2-(4-METHYL-THIAZOL-5-YL)-ETHANOL | C6 H9 N O S | 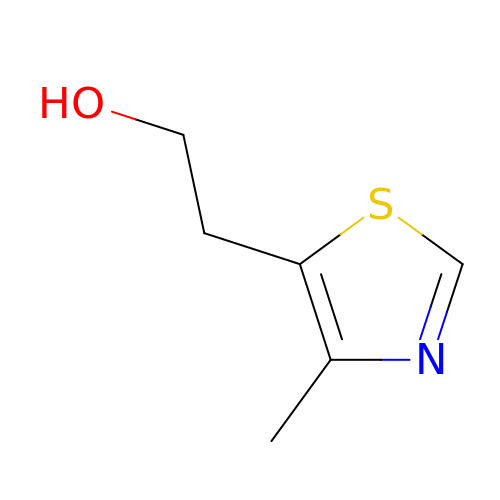BKAWJIRCKVUVED-UHFFFAOYSA-N>GPKVPEFGSSRIDALEYATTRKKSEVVYSGVSVTIPTAPTNLVSLLKTLTPSSGTLAPFFDTVNNKMVVFNENKTLFFKLSIVGTWPSGTANRSMQLTFSGSVPDTLVSSRNSATTTDNILLATF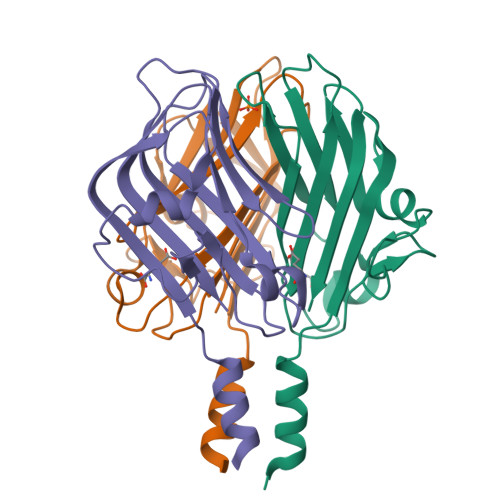FSVDKDGFLATNGSTLTIQSNGASFTATTIKIIAEQ[3x]> DEHCERLPYDASKWEFPRDRLKLGKPLGRGAFGQVIEADAFGIDKTATCRTVAVKMLKEGATHSEHRALMSELKILIHIGHHLNVVNLLGACTKPGGPLMVIVEFCKFGNLSTYLRSKRNEFVPYKVAPEDLYKDFLTLEHLICYSFQVAKGMEFLASR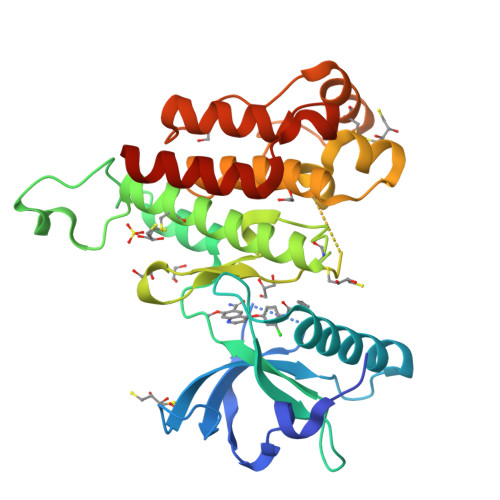KCIHRDLAARNILLSEKNVVKICDFGLARDIYKDPDYVRKGDARLPLKWMAPETIFDRVYTIQSDVWSFGVLLWEIFSLGASPYPGVKIDEEFCRRLKEGTRMRAPDYTTPEMYQTMLDCWHGEPSQRPTFSELVEHLGNLLQANAQQDG>[6x]MIPVTELRYFADTQPAYRILKPWWDVFTDYISIVMLMIAVFGGTLQVTQDKMICLPCKWVTKDSCNDSFRGWAASSPEPTYPNSTVLPTPDTGPTGIKYDLDRHQYNYVDAVCYENRLHWFAKYFPYLVLLHTLIFLACSNFWFKFPRTSSKLEHFVSILLKCFDS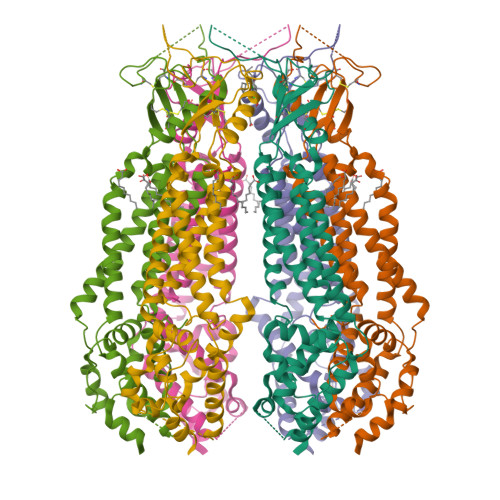PWTTRALSETVVEESDPKPAFSKMNGSMDKKSSTVSEDVEATVPMLQRTKSRIEQGIVDRSETGVLDKKEGEQAKALFEKVKKFRTHVEEGDIVYRLYMRQTIIKVIKFALIICYTVYYVHNIKFDVDCTVDIESLTGYRTYRCAHPLATLFKILASFYISLVIFYGLICMYTLWWMLRRSLKKYSFESIREESSYSDIPDVKNDFAFMLHLIDQYDPLYSKRFAVFLSEVSENKLRQLNLNNEWTLDKLRQRLTKNAQDKLELHLFMLSGIPDTVFDLVELEVLKLELIPDVTIPPSIAQLTGLKELWLYHTAAKIEAPALAFLRENLRALHIKFTDIKEIPLWIYSLKTLEELHLTGNLSAENNRYIVIDGLRELKRLKVLRLKSNLSKLPQVVTDVGVHLQKLSINNEGTKLIVLNSLKKMVNLTELELIRCDLERIPHSIFSLHNLQEIDLKDNNLKTIEEIISFQHLHRLTCLKLWYNHIAYIPIQIGNLTNLERLYLNRNKIEKIPTQLFYCRKLRYLDLSHNNLTFLPADIGLLQNLQNLAVTANRIEALPPELFQCRKLRALHLGNNVLQSLPSRVGELTNLTQIELRGNRLECLPVELGECPLLKRSGLVVEEDLFSTLPPEVKERLWRADKEQASNSLEVLFQG The bacterial pLGIC from Gloeobacter violaceus (GLIC) is a cationic homo-pLGIC. The crystal structures of GLIC show a common scaffold with the vertebrate pLGICs, such as nicotinic acetylcholine receptors (nAChRs), except without an IC domain. Opening of the GLIC channel is triggered by extracellular protons, but it is unclear which titratable residues are responsible for the GLIC activation. Vertebrate pentameric ligand-gated ion channels (pLGICs) regulate ionic conductance in nerve cells and play an important role in fast synaptic signal transduction. They are formed by five homologous or identical subunits assembled around the central channel axis.

The first one is at the C loop region, where residues E177, D178, and R179 potentially form salt bridges with residues K148 and D91 at the complementary site of an adjacent subunit. We performed mutations (D91N, E177Q, and D178N, termed the NQN mutation) to remove the potential of salt bridges. The overall structures of the NQN mutant and GLIC are nearly the same (RMSD ∼0.5 Å) and show an open channel conformation. However, the C loop of the NQN mutant shows an outward movement and the interfacial gap in the C loop region, measured by side chain displacement of D178N, widens 3 Å. The NQN mutation removed the salt bridges but did not generate hydrogen bonds. The resultant free energies of –29 kcal/mol and –26 kcal/mol for GLIC and the NQN mutant, respectively, suggest that removing the salt bridges at the subunit interface destabilized the open channel conformation. The mutation shifted the EC50 from pH 5.0 in the wild type GLIC to pH 4.8 in the NQN mutant. Apparently, more protons are required for channel activation to compensate for destabilization of the open-channel conformation due to the absence of the inter-subunit salt bridges. The pertubation originated from the NQN mutation site was transmitted immediately to Y23, L103, R133, and K148. Among them, R133 and K148 form intra- and inter-subunit salt bridges with D178 and E177, respectively.

>GQDMVSPPPPIADEPLTVNTGIYLIECYSLDDKAETFKVNAFLSLSWKDRRLAFDPVRSGVRVKTYEPEAIWIPEIRFVNVENARDADVVNISVSPDGTVQYLERFSARVLSPLDFRRYPFDSQTLHIYLIVRSVDTRNIVLAVDLEKVGKNDDVFLTGWDIESFTAVVKPANFALQNRLESKLDYQLRISRQYFSYIPNIILPMLFILFISWTAFWSTSYEANVTLVVSTLIAHIAFNILVETNLPKTPYMTYTGAIIFMIYLFYFVAVIEVTVQHYLKVESQPARAASITRASRIAFPVVFLLANIILAFLFFGF[5x]>[12x]GGSMSKTIVLSVGEATRTLTEIQSTADRQIFEEKV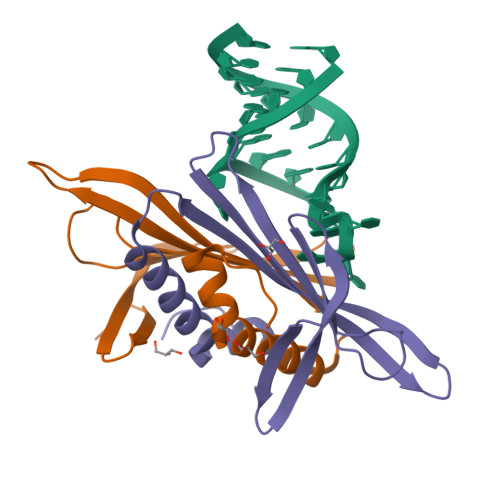GPLVGRLRLTASLRQNGAKTAYRVNLKLDQADVVDSGLPKVRYTQVWSHDVTIVANSTEASRKSLYDLTKSLVATSQVEDLVVNLVPLGR> MSLSLFGVKNNWHKNGIWWFSKILNKTVGEERYDALRVQRRIWSMRFYYARQQCLYELFVDHPDLAQWTGTYPKVDSSHGFPFYSTYEMYRDFQENTLNSDGSFAQWITLVCGIYVIHVIYNYMIPYYWVSTPLKNDEFTRLRMKDYIASTVLEEVYGISYAEWGWLPHDFAYNRMRGLAGYMHPDDPRAMCTSTFHRKHKYIEHEVEKVGDYHHM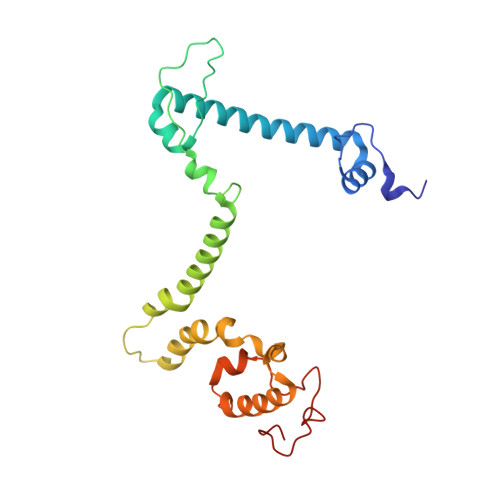TYPK> MEQEKIRIKLRAYDHRLLDQSVKQIIET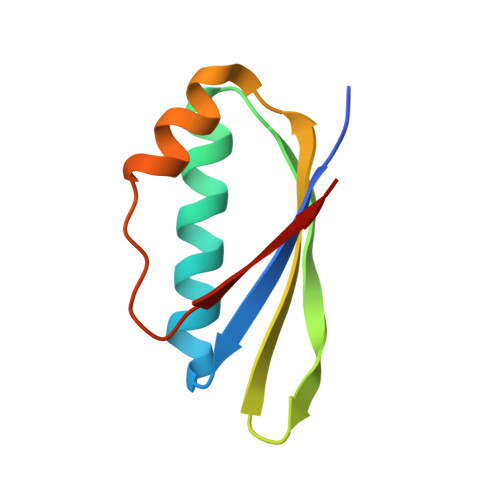VKRTGGVVKGPIPLPTRKSEFSRILDIIRFTPQTIEALMEISLPAGVDVEVKMRG> SSRVIVHVDLDCFYAQVEMISNPELKDKPLGVQQKYLVVTCNYEARKLGVKKLMNVRDAKEKCPQLVLVNGEDLTRYREMSYKVTELLEEFSPVVERLGFDENFVDLTEMVEKRLQQLQSDELSAVTVSGHVYNNQSINLLDVLHIRLLVGSQIAAEMREAMYNQLGLTGCAGVASNKLLAKLVSGVFKPNQQTVLLPESCQHLIHSLNHIKEIPGIGYKTAKCLEALGINSVRDLQTFSPKILEKELGISVAQRIQKLSFGEDNSPVILSGPPQSFSEEDSFKKCSSEVEAKNKIEELL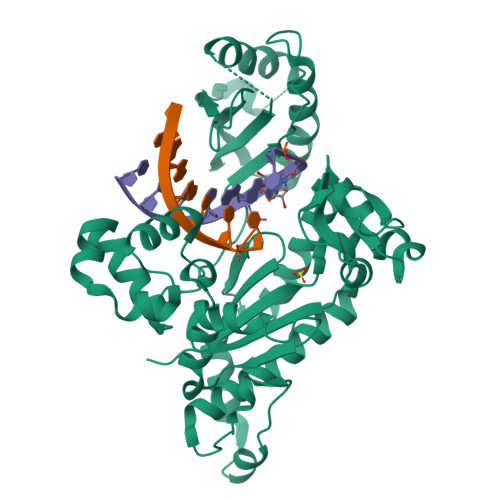ASLLNRVCQDGRKPHTVRLIIRRYSSEKHYGRESRQCPIPSHVIQKLGTGNYDVMTPMVDILMKLFRNMVNVKMPFHLTLLSVCFCNLK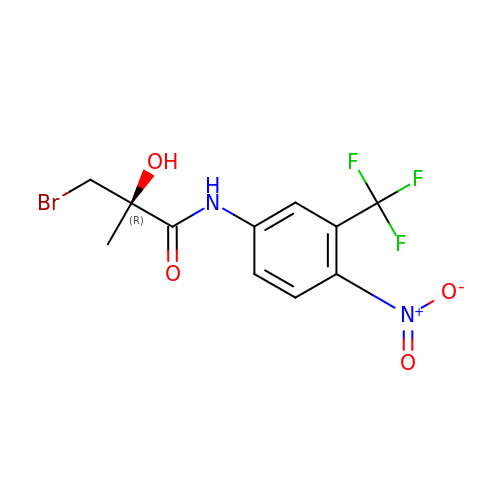(R)-3-BROMO-2-HYDROXY-2-METHYL-N-[4-NITRO-3-(TRIFLUOROMETHYL)PHENYL]PROPANAMIDE | C11 H10 Br F3 N2 O4 | QDSWNDMHSBZXKX-JTQLQIEISA-N>[2x]SNAMANFEDFLTLDL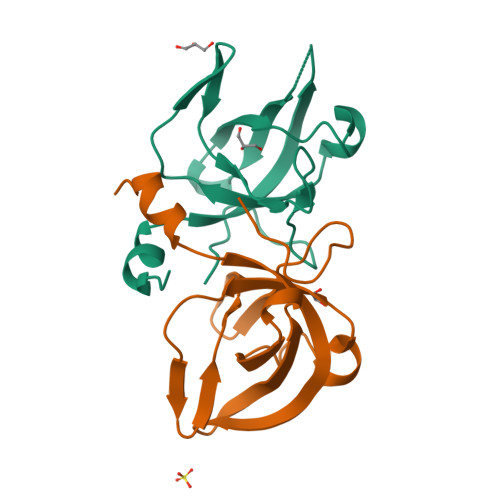RIGTVTHAEEFKEARVPAIRLEIDFGELGMKQSSAQITKRYNPEDLIGQQIVAVVNFPPKRVAGFKSEVLVLGGVPEAGDVVLLQPNMELPNGTKIS>[3x]MTQQIKYKRVLLKLSGESLMGSDPFGINHDTIVQTVGEIAEVVKMGVQVGIVVGGGNIFRGVSAQAGSMDRATADYMGM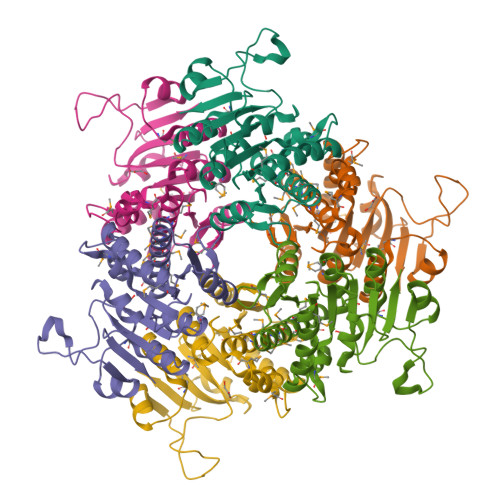MATVMNALALKDAFETLGIKARVQSALSMQQIAETYARPKAIQYLEEGKVVIFAAGTGNPFFTTDTAAALRGAEMNCDVMLKATNVDGVYTADPKKDPSATRYETITFDEALLKNLKVMDATAFALCRERKLNIVVFGIAKEGSLKRVITGEDEGTLVHC> MLVAYDSMTGN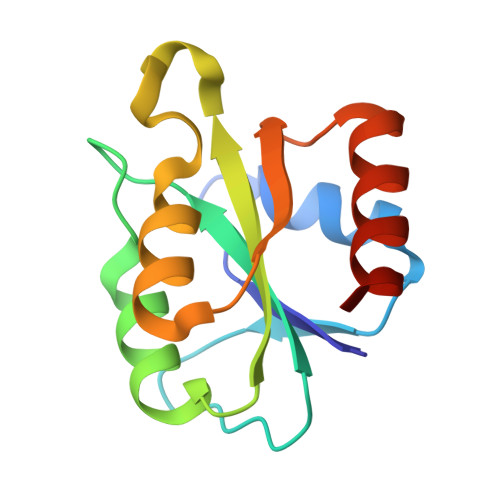VKRFIHKLNMPAVQIDEDLVIDEDFILITYTTGFGNVPERVLDFLERNNEKLKGVSASGNRNWGDMFGASADKISTKYEVPIVSKFELSGTNNDVEYFKERVREIATH>MASQPNSSAKKKEEKGKNIQVVVRCRPFNLAERKASAHSIVECDPVRKEVSVRTGGLADKSSRKTYTFDMVFGASTKQIDVYRSVVCPILDEVIMGYNCTIFAYGQTGTGKTFTMEGERSPNEEYTWEEDPLAGIIPRTLHQIFEKLTDNGTEFSVKVSLLEIYNEELFDLLNPSSDVSERLQMFDDPRNKRGVIIKGLEEITVHNKDEVYQILEKGAAKRTTAATLMNAYSSRSHSVFSVTIHMKETTIDGEELVKIGKLNLVDLAGSENIGRSGAVDKRAREAGNINQSLLTLGRVITALVERTPHVPYRESKLTRILQDSLGGRTRTSIIATISPASLNLE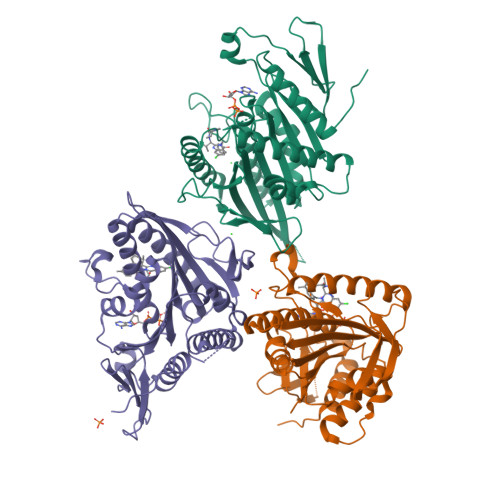ETLSTLEYAHRAKNILNKPEVNQK[3x]>MPSLMSFGSCQWIDQGRFSRSLYRNFKTFKLHEMHGLCMPNLLLNPDIHGDRIIFVCCDDLWEHDLKSGSTRKIVSNLGVINNARFFPDGRKIAIRVMRGSSLNTADLYFYNGENGEIKRITYFSGKSTGRRMFTDVAGFDPDGNLIISTDAMQPFSSMTCLYRVENDGINFVPLNLGPATHILFADGRRVIGRNTFELPHWKGYRGGTRGKIWIEVNSGAFKKIVDMSTHVSSPVIVGHRIYFITDIDGFGQIYSTDLDGKDLRKHTSFTDYYPRHLNTDGRRILFSKGGSIYIFNPDTEKIEKIEIGDLESPEDRIISIPSKFAEDFSPLDGDLIAFVSRGQAFIQDVSGTYVLKVPEPLRIRYVRRGGDTKVAFIHGTREGDFLGIYDYRTGKAEKFEENLGNVFAMGVDRNGKFAVVANDRFEIMTVDLETGKPTVIERSREAMITDFTISDNSRFIAYGFPLKHGETDGYVMQAIHVYDMEGRKIFAATTENSHDYAPAFDADSKNLYYLSYRSLDPSPDRVVLNFSFEVVSKPFVIPLIPGSPNPTKLVPRSMTSEAGEYDLNDMYKRSSPINVDPGDYRMIIPLESSILIYSVPVHGEFAAYYQGAPEKGVLLKYDVKTRKVTEVKNNLTDLRLSADRKTVMVRKDDGKIYTFPLEKPEDERTVETDKRPLVSSIHEEFLQMYDEAWKLARDNYWNEAVAKEISERIYEKYRNLVPLCKTRYDLSNVIVEMQGEYRTSHSYEMGGTFTDKDPFRSGRIACDFKLDGDHYVVAKAYAGDYSNEGEKSPIFEYGIDPTGYLIEDIDGETVGAGSNIYRVLSEKAGTSARIRLSGKGGDKRDLMIDILDDDRFIRYRSWVEANRRYVHERSKGTIGYIHIPDMGMMGLNEFYRLFINESSYQGLIVDVRFNGGGFVSQLIIEKLMNKRIGYDNPRRGTLSPYPTNSVRGKIIAITNEYAGSDGDIFSFSFKKLGLGKLIGTRTWGGVVGITPKRRLIDGTVLTQPEFAFWFRDAGFGVENYGVDPDVEIEYAPHDYLSGKDPQIDYAIDALIEELRNW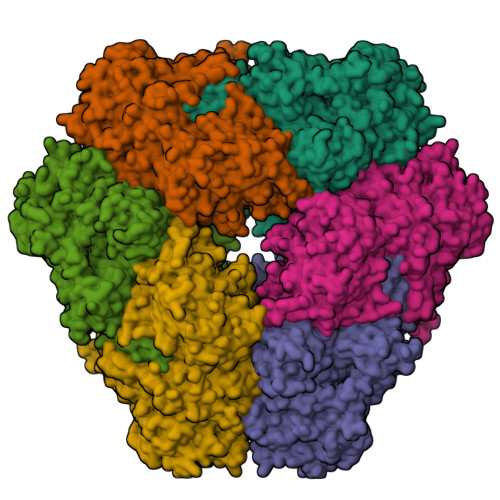NEELPQRPS[6x]> IIGGRESRPHSRPYMAYLQIQSPAGQSRCGGFLVREDFVLTAAHCWGSNINVTLGAHNIQRRENTQQHITARRAIRHPQYNQRTIQNDIMLLQLSRRVRRNRNVNPVALPRAQEGLRPGTLCTVAGWGRVSMRRGTDTLREVQLRVQRDRQCLRIFGSYDPRRQICVGDRRERKAAFK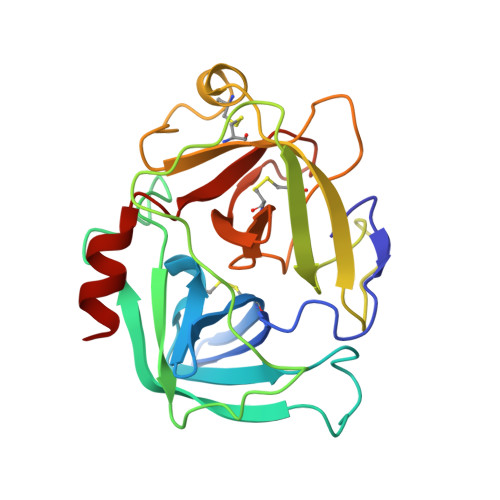GDSGGPLLCNNVAHGIVSYGKSSGVPPEVFTRVSSFLPWIRTTMR N-[(6-bromo-1H-indol-1-yl)acetyl]glycine | C12 H11 Br N2 O3 | 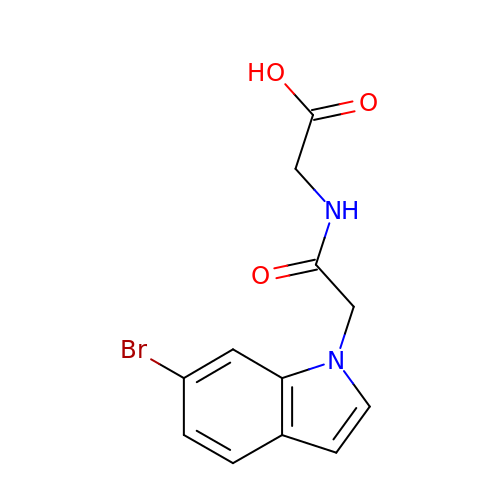CWLHYPMSORHOPU-UHFFFAOYSA-N>MNQHSHKDYETVRIAVVRARWHADIVDQCVSAFEAEMADIGGDRFAVDVFDVPGAYEIPLHARTLAETGRYGAVLGTAFVVNGGIYRHEFVASAVIDGMMNVQLSTGVPVLSAVLTPHNYHDSAEHHRFFFEHFTVKGKEAARAC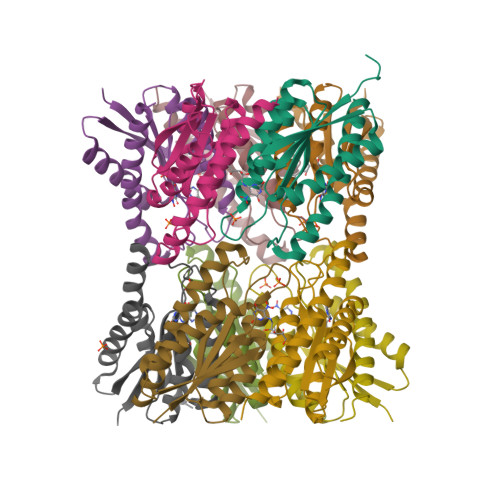VEILAAREKIAA[10x]>YAHHPIDYERSTSKSPNILRLPANTSDPTYQENMARMEGLVEQLRARVRYVQAGGVVPEEEAAKAGVSISSIEADDRVRKLHLSRGKMLARDRIERLIDPGTRFLELSQLAGWDLYWDDKKKEYERCYSGGIVTGIGLVNGVRCMLVANDATVKGGTYYPITVKKHLRAQKIAEQNHLPCIYLVDSGGANLSRQDDVFPDEQHFGRIFYNEAQMSIKSISQIAVVMGSCTAGGAYVPAMADENIIVARNGTIFLGGPPLVLAATGEKVSSEELGGADVHCRISGVGDHYATDDLHALYLARRAVANLNLKEHNEARNPTDVKPVPPLYDPRELGGFIPDMLSDVVKSFDVRAIIARIVDGSRFDEFKALYGNTLVCGFARIEGMQVGIIANQGILYSESALKGAHFIGLCTQRNVPLLFLQNITGFMVGKKYEEGGIARNGARLVMAVSSAPVPKVTVLIGGSYGAGNYGMCGRAFEPRFLFMWPNARISVMGGTQAATVLTLTNRNLKNASEAEIAAFKDKVKKKYEKEGSCYYSTARLWDDGVIAPEDTRVVVAEALRATRLAP[6x];>[6x]ERKVEKLLVANRGEIACRVFRTCREMHIRTVALFCEAERNAKHVAEADEAVCIGPPPAVNSYLRGEHIISVAKQLNVDAIHPGYGFLSENASFADAITRSGIEFIGPPASAISLMGSKSESKRIMEAAGVPVVPGYYGENQNVSFLAEEAKKVGFPILIKAVSGGGGKGMKIVERPEDFTFMLESAKREATNFFKDDRVILERYVKRSRHIECQIFFDKHGRGVFFFERDCSVQRRYQKVLEEAPAPHLSMETRQRIGEVALQAAKAVGYVGAGTVEFIFDTSTGEFYFMEMNTRLQVEHPVTEEVCRIKGAPLDLVKLQIKTAMGKPLTFSQEDVTLVGSCIEARVYAESPERGFLPESGPLTFIREPFQGVRGPARTRLDTGFREGDNVLIHYDPMLAKVISWGRSREEALRGLRQALGEYKVAGINTNIEFLKRCCETPEFARGGVTTNFISEHESQLLKSPVVTPEVAAMAATAWLLNRCDNWRGAFRLNSDTNATVHFYIDDHPVEVRLHTEGANYHKIFFSVWDHDGSFEVCSGPVTSKHRDQKSIVNDFTFLFENGMHHTVLAVATEGDVTVIGSFGLHQLRLLPLTDGFGDSST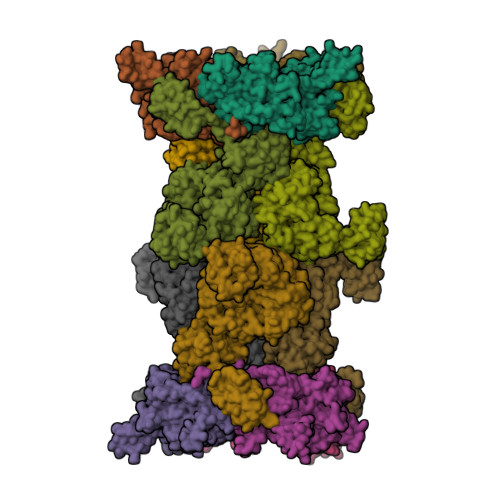AGGTSTKIVSPMPGKVSKLLVKSGDLVEKGQVLVIVEAMKMEHPVRALQDGRVSFLVKEGEVVGGDHVLATVAEEE>MGSDKIHHHHHHMKKLTVYLATTNPHKVEEIKMIAPEWMEILPSPEKIEVVEDGETFLENSVKKAVVYGKKLKHPVMADDSGLVIYSLGGFPGVMSARFMEEHSYKEKMRTILKMLEGKDRRAAFVCSATFFDPVENTLISVEDRVEGRIANEIRGTGGFG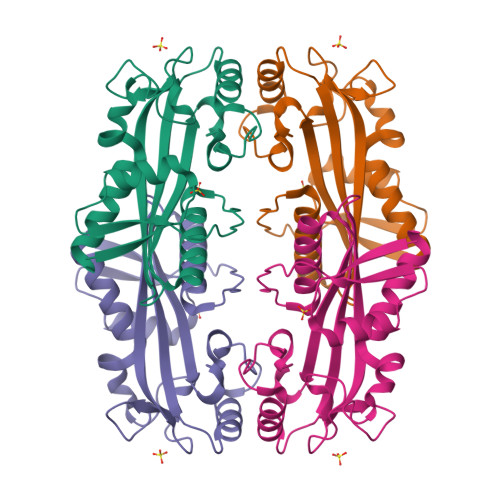YDPFFIPDGYDKTFGEIPHLKEKISHRSKAFRKLFSVLEKILESENR[2x]3,4,5-trihydroxybenzoic acid | C7 H6 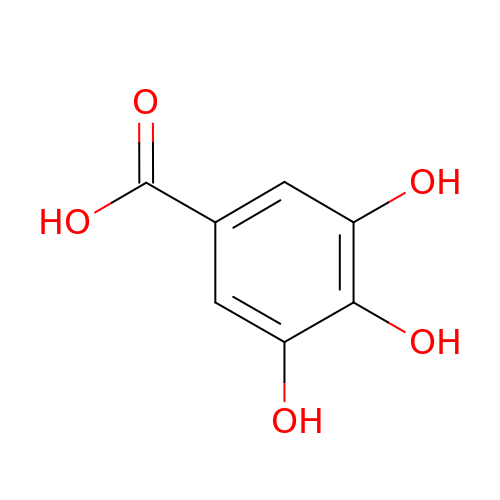O5 | LNTHITQWFMADLM-UHFFFAOYSA-N> GSHMSQSNRELVVDFLSYKLSQKGY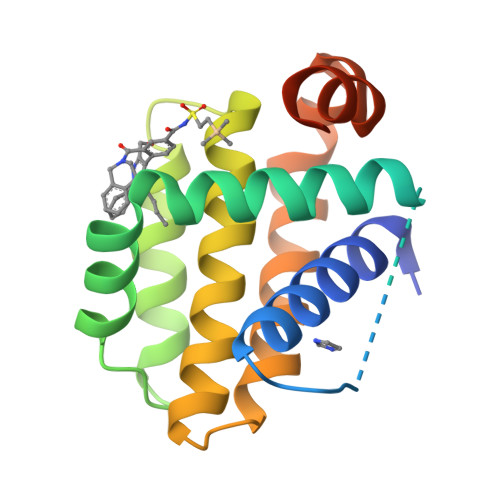SWSQFSDVEENRTEAPEGTESEAVKQALREAGDEFELRYRRAFSDLTSQLHITPGTAYQSFEQVVNELFRDGVNWGRIVAFFSFGGALCVESVDKEMQVLVSRIAAWMATYLNDHLEPWIQENGGWDTFVELYGNNAAAESRKGQER> LEAELHNCVVVQFDGPMSFYVQMESDVPALEQMTDKLLDAEQDLPAFSDLKEGALCVAQFPEDEVFYRAQIRKVLDDGKCEVHFIDFGNNAVTQQFRQLPEELAKPARYSRHCELDASTISKCDA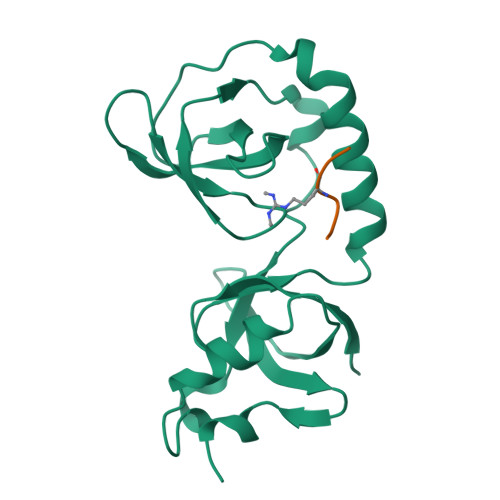ALLQSFIDTRFSETFQVEILATKGTGTHVVRLFYQSKNISEKLQECQ;> ARGRGR1-[4-[(1~{R})-1-[2-[[5-[1-(cyclopropylmethyl)pyrazol-4-yl]-1~{H}-benzimidazol-2-yl]amino]pyridin-4-yl]ethyl]piperazin-1-yl]-3,3,3-tris(fluoranyl)propan-1-one 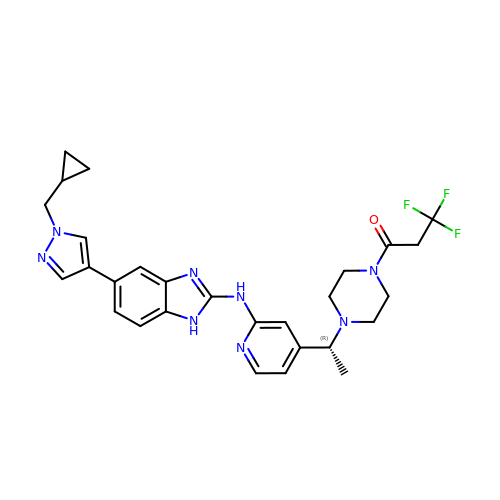| C28 H31 F3 N8 O | WEFRCKPVMWDRAK-GOSISDBHSA-N> ADPASEEVMACLRQERSRVENPSQTIVNVVAENPAYLHCSVPPDAEHEIAWTRVSDGALLTAGNRTFTRDPRWQVSKKSANIWVLNLRRAEQQDSGCYLCEIN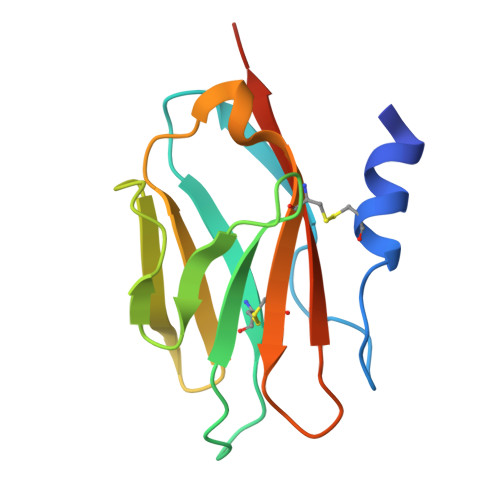DKHNTVYAVYLKVLEPHHHHHH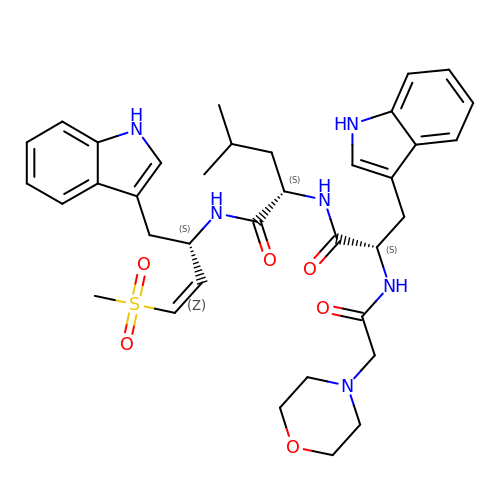(2S)-N-[(E,2S)-1-(1H-indol-3-yl)-4-methylsulfonyl-but-3-en-2-yl]-2-[[(2S)-3-(1H-indol-3-yl)-2-(2-morpholin-4-ylethanoylamino)propanoyl]amino]-4-methyl-pentanamide | C36 H46 N6 O6 S | AZZZSQJQBKRGDX-LGBXHZPNSA-N> GEIT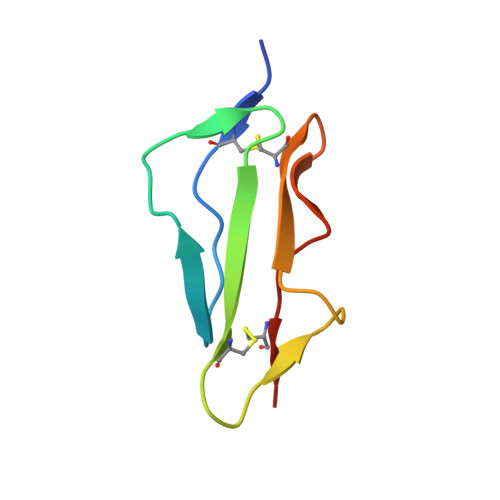CDPPRIPNGVYRPELSKYRGQDKITYECKKGFFPEIRGTDATCTRDGWVPVPRCAWK>[2x]MGPGFDFAQAIMKKNTVIARTEKGEFTMLGVYDRVAVIPTHASVGEIIYINDVETRVLDACALRDLTDTNLEITIVKLDRNQKFRDIRHFLPRCEDDYNDAVLSVHTSKFPNMY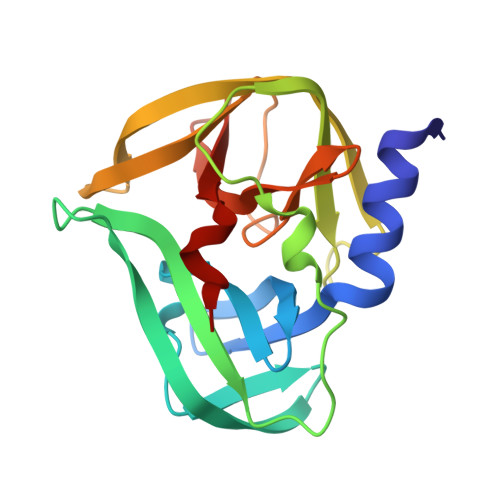IPVGQVTNYGFLNLGGTPTHRILMYNFPTRAGQCGGVVTTTGKVIGIHVGGNGAQGFAAMLLHSYFTD> MSEFLTPERTVYDSGVQ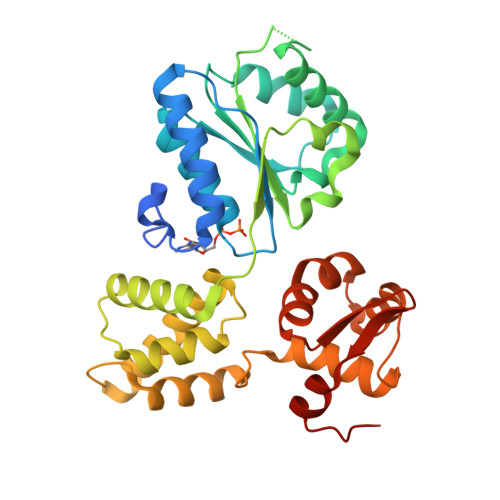FLRPKSLDEFIGQENVKKKLSLALEAAKMRGEVLDHVLLAGPPGLGKTTLAHIIASELQTNIHVTSGPVLVKQGDMAAILTSLERGDVLFIDEIHRLNKAVEELLYSAIEDFQIDIMIGKGPSAKSIRIDIQPFTLVGATVRSGLLSSPLRSRFGIILELDFYTVKELKEIIKRAASLMDVEIEDAAAEMIAKRSRGTPRIAIRLTKRVRDMLTVVKADRINTDIVLKTMEVLNIDDEGLDEFDRKILKTIIEIYRGGPVGLNALAASLGVEADTLSEVYEPYLLQAGFLARTPRGRIVTEKAYKHLKYEVPENRLF>[2x]GGACCUCGGCGAAAGCCGUUCGACCAGCGAAAGCUCUUAGACAGGAGGUUAG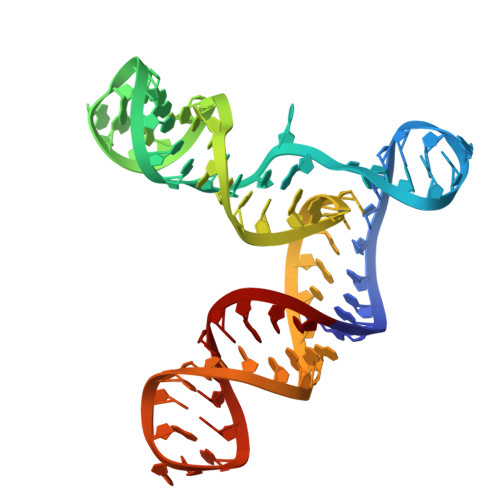GUGCUCCGAAAGGAGCACU Syntenin is a small intracellular scaffold protein that contains two PSD‐95, Discs‐large, ZO‐1 (PDZ) domains that bind SDC, an N‐terminal domain that binds ALIX (via three LYPxL motifs), and a short C‐terminal domain regulating the conformation of the protein and accessibility of its domains (Baietti et al., 2012; Grootjans et al., 1997; Saito, Nishioka, Iwatsuki, Kumagai, & Sasaki, 1975). The PDZ domains of syntenin bind the C‐termini of the SDCs (Grootjans et al., 1997), but bind also to PIP2 (Zimmermann et al., 2002) and several other membrane proteins, including CD63 (Latysheva et al., 2006). In contrast, SDC‐syntenin‐ALIX binding regulates the formation of endosomal intraluminal vesicles and the secretion of CD63+ exosomes that contain syntenin, C‐terminal fragments of the SDCs (SDC‐CTFs) and potential SDC‐cargo such as ligand‐engaged receptors (Baietti et al., 2012). Since syntenin activity strictly depends on the functionality of its PDZ domains (Baietti et al., 2012; Grootjans et al., 1997; Grootjans, Reekmans, Ceulemans, & David, 2000; Koo et al., 2002; Lambaerts et al., 2012; Luyten et al., 2008; Meerschaert et al., 2007; Zimmermann et al., 2002; Zimmermann et al., 2005; Zimmermann et al., 2001), we aimed to develop syntenin PDZ inhibitors and investigate their potential utility to control cellular phenotypes as well as exosomal‐releases.

Five structurally related compounds (valine–like analogues mimicking the last hydrophobic residue of a PDZ binding motif), namely C4, C37, C38, C47 and C58 were identified to inhibit syntenin PDZ interactions while having no significant effect on control (biotinylated‐GST) FRET signals. The C58 inhibitor was selected for further investigations because it yielded the highest extinction of the HTRF signal. To validate and characterize the binding mode of the most potent compound C58 with its target protein, syntenin crystals were soaked with the compound. The phenyl ring of fragment C58 shows a strong face‐to‐face π‐stacking with Phe213, its nitrogen atom making a hydrogen‐bonding interaction with the backbone carbonyl of Phe211 and its carboxylic acid making the expected canonical hydrogen‐bonding interactions with the backbone nitrogen of Val209, Gly210 and Phe211. Moreover, co‐crystallization experiments indicated that C58 binds syntenin PDZ2 but not PDZ1 domain. C58 was further characterized in dose‐response HTRF assays testing syntenin‐SDC2 interaction and the IC50 was determined to be 350 µM. The binding of C58 to syntenin was also validated in surface plasmon resonance experiments (BIAcore) and in this experimental setting apparent KD values were determined to be 886 µM and 1026 µM for syntenin‐PDZ tandem plus C‐terminal domain and syntenin‐PDZ tandem (without C‐terminal domain) respectively. Consistent with the selectivity of C58 for syntenin, no binding could be observed in BIAcore between this compound and GRASP55‐PDZ tandem.

>[4x]GAMDPREVILCKDQDGKIGLRLKSIDNGIFVQLVQANSPASLVGLRFGDQVLQINGENCAGWSSDKAHKVLKQAFGEKITMTIRDRPFERTITMHKDSTGHVGFIFKNGKITSIVKDSSAARNGLLTEHNICEINGQNVIGLKDSQIADILSTSGTVVTITIMPAF>[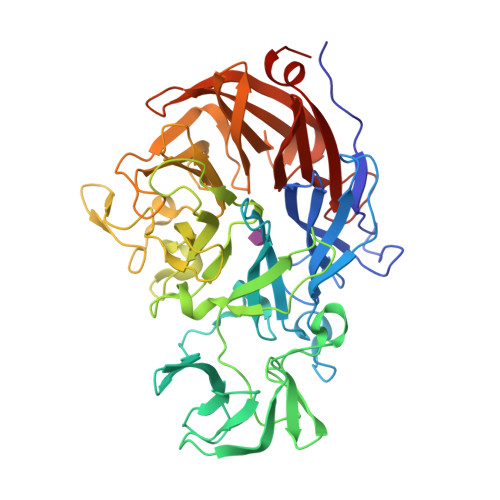2x]LPEGAALTEKTDIFESGRNGKPNKDGIKSYRIPALLKTDKGTLIAGADERRLHSSDWGDIGMVIRRSEDNGKTWGDRVTITNLRDNPKASDPSIGSPVNIDMVLVQDPETKRIFSIYDMFPEGKGIFGMSSQKEEAYKKIDGKTYQILYREGEKGAYTIRENGTVYTPDGKATDYRVVVDPVKPAYSDKGDLYKGNQLLGNIYFTTNKTSPFRIAKDSYLWMSYSDDDGKTWSAPQDITPMVKADWMKFLGVGPGTGIVLRNGPHKGRILIPVYTTNNVSHLNGSQSSRIIYSDDHGKTWHAGEAVNDNRQVDGQKIHSSTMNNRRAQNTESTVVQLNNGDVKLFMRGLTGDLQVATSKDGGVTWEKDIKRYPQVKDVYVQMSAIHTMHEGKEYIILSNAGGPKRENGMVHLARVEENGELTWLKHNPIQKGEFAYNSLQELGNGEYGILYEHTEKGQNAYTLSFRKFNWDFLSKDL> TLSLANYLAADSAAEALRRDVRAGLTAAPKSLPPKWFYDAVGSDLFDQITRLPEYYPTRTEAQILRTRSAEIIAAAGADTLVELGSGTSEKTRMLLDAMRDAELLRRFIPF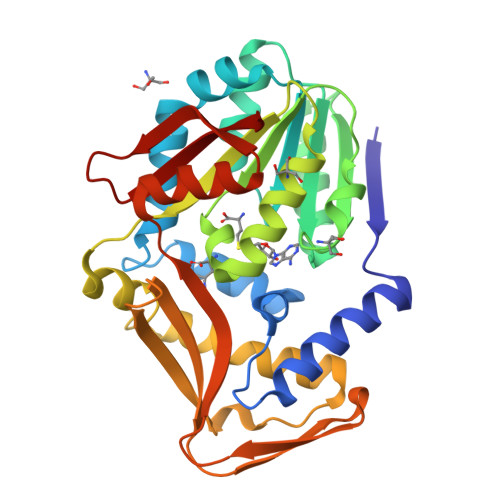DVDAGVLRSAGAAIGAEYPGIEIDAVCGDFEEHLGKIPHVGRRLVVFLGSTIGNLTPAPRAEFLSTLADTLQPGDSLLLGTDLVKDTGRLVRAYDDAAGVTAAFNRNVLAVVNRELSADFDLDAFEHVAKWNSDEERIEMWLRARTAQHVRVAALDLEVDFAAGEEMLTEVSCKFRPENVVAELAEAGLRQTHWWTDPAGDFGLSLAVRL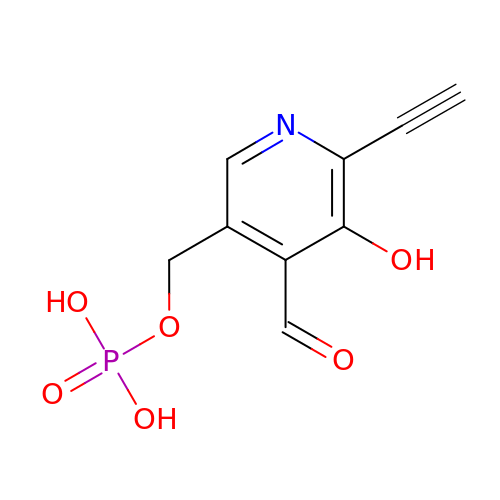(6-ethynyl-4-methanoyl-5-oxidanyl-pyridin-3-yl)methyl dihydrogen phosphate | C9 H8 N O6 P | OAIRLJMOEFCXML-UHFFFAOYSA-N>[2x]VAESKLVIGDRSFASRLIMGTGGATNLAVLEQALIASGTELTTVAIRRVDADGGTGLLDLLNRLGITPLPNTAGSRSAAEAVLTAQLAREALNTNWVKLEVIADERTLWPDAVELVRAAEQLVDDGFVVLPYTTDDPVLARRLEDTGCAAVMPLGSPI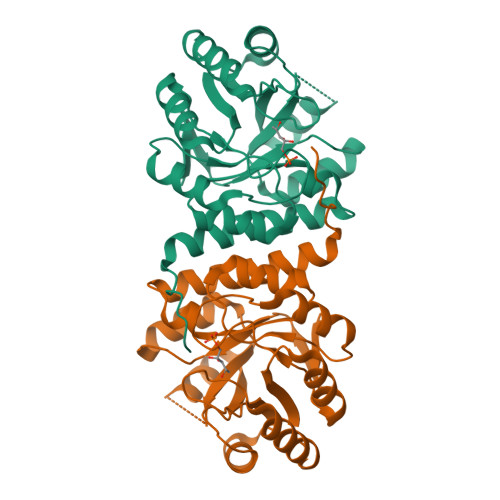GTGLGIANPHNIEMIVAGARVPVVLDAGIGTASDAALAMELGCDAVLLASAVTRAADPPAMAAAMAAAVTAGYLARCAGRIPKRFWAQASSPAR>[3x]MEGQRDSAFPKFESKP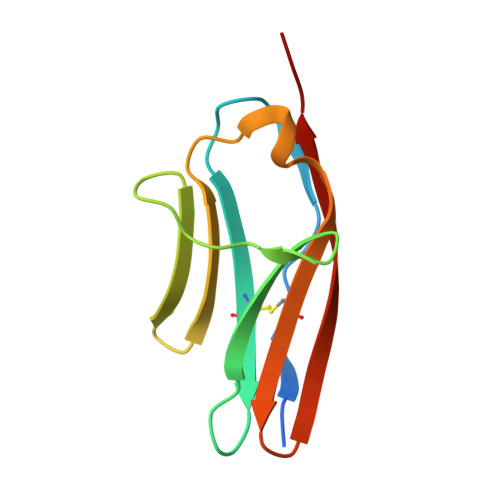QSQEVKENQTVKFRCEVSGIPKPEVAWFLEGTPVRRQEGSIEVYEDAGSHYLCLLKARTRDSGTYSCTASNAQGQLSCSWTLQVERL BENZHYDROXAMIC ACID | C7 H7 N O2 | 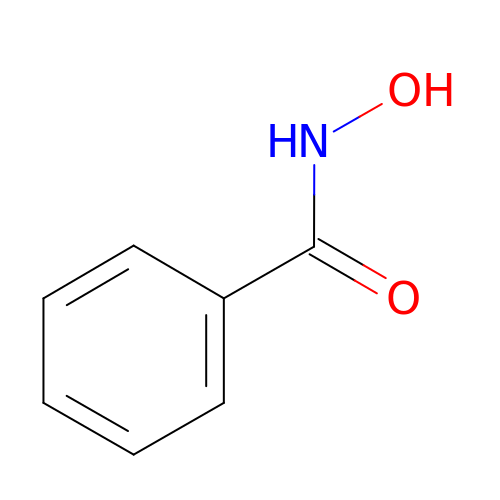VDEUYMSGMPQMIK-UHFFFAOYSA-N> STQKSLSKEEIERYSRQMIVPGMGKEGQLRLMNAKVLIIGAGGLGCPAAQYLAGAGVGTIGIVDGDSVETSNLHRQVAHATKRVGM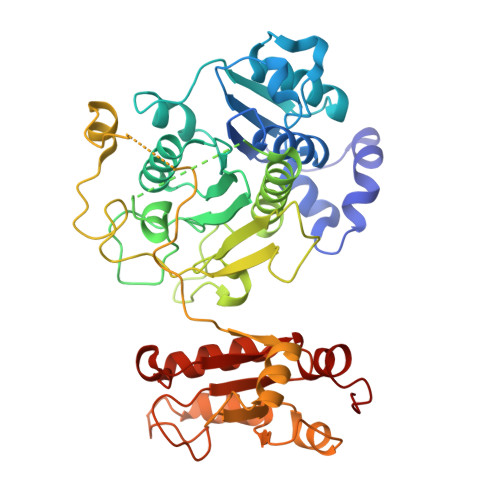LKVDSLITHLIEINPLPVYVPYRFDLTPQNAAQIIKPWDVILDCTDNPATRYLISDVCVLLGKPLVSAASVQKSGQLIVLNCPPTPQGVVNKKAAPCYRCCFKKPPPPSAQTSCGEAGIMGPVVGMMGVAQAGEAIKILVSQLHMPPKEGEEVSPEKNLVQPTLLIYTYDLNSAIGPYSFRALKMGGRKKDCFACGENSTLTLDGIKSGNPNYVQFCGNMTQSTNLAPEDRITATAYNEKRRNGELGEHILLDTREKEHFSFGSIPGAVNVPFSKFLVKASSIKREGNSPAELLPMQPASDEAPIVVVCRRGQDSQEVVEKLKELGLDNGGKRKIMDIVGGMKAWRDEVDPDFPFI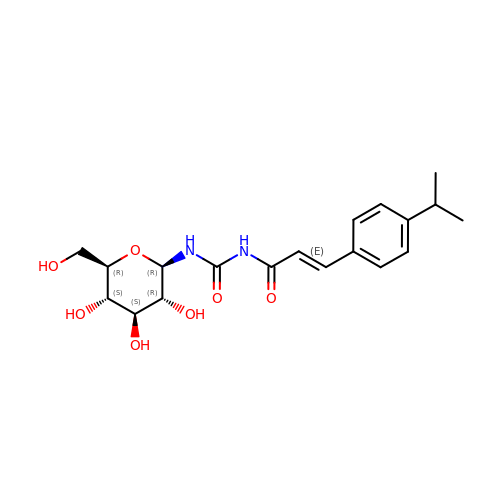N-({(2E)-3-[4-(propan-2-yl)phenyl]prop-2-enoyl}carbamoyl)-beta-D-glucopyranosylamine | C19 H26 N2 O7 | RIYKPZZUXJMBTL-AWRGUQPNSA-N5-iodo-1H-pyrazole 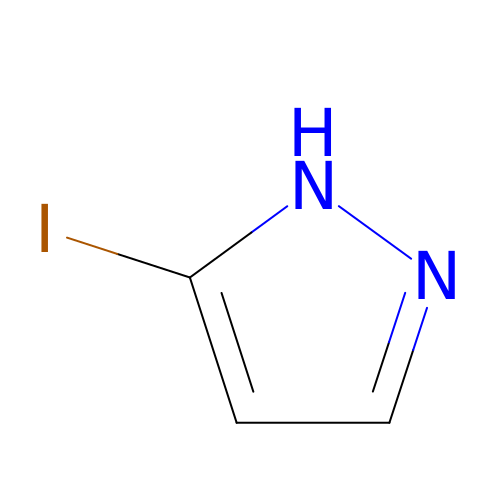| C3 H3 I N2 | RUKDVLFJSMVBLV-UHFFFAOYSA-N The Aerococcus viridans L-lactate oxidase (avLOX) is a biotechnologically important member of this flavoenzyme family and it catalyzes oxidation of L-lactate and O2 into pyruvate and H2O2. Common characteristics of their structure are the (β/α)8 barrel fold and arrangement of protein subunits into a functional homotetramer2. The FMN is bound at the C-terminal end of the internal β barrel. A special and interesting feature of the catalytic center of avLOX is that it contains a third tyrosine (Tyr215), which forms a weak hydrogen bond with the pyruvate O2 in the wild-type structure.

Crystals of the Y215F mutant grew in the P21 spacegroup and had two tetramers within the asymmetric unit. Also present in each subunit is the FMN cofactor and a pyruvate which both bind in a similar manner to the wild-type enzyme. Residues 200–215 in subunit D and 200–216 in subunit H, which reside in loop 4 had no corresponding interpretable density. These residues form a short helical structure, which could function as an active-site lid, and residues near this range have been observed to be disordered in other structures suggesting an inherent mobility. In the six subunits with observable loop residues, the pyruvate is bound in a manner very similar to the wild-type enzyme except for a difference in the interaction with the amino acid at position 215. The interaction in the enzyme variant positions the nearest Phe215 ring atom within ~3.5 Å of the pyruvate methyl group to replace the hydrogen bond with a hydrophobic interaction. The hydrogen bond with Arg181 is also lost. In the two subunits without observable density for the loop, the pyruvate maintains some of the interactions between its carboxylate and Arg268 and Arg181 but shifts in the pyruvate and both of these side chains result in weaker interactions. The k5 of Y215F (20.3 s−1) at pH 6.5 was lowered 7-fold compared to the corresponding k5 of the wild-type enzyme (141 s−1). Evidence that k5 was nevertheless slowed down in the Y215F variant compared to wild-type enzyme at pH 6.5 could be explained by the development of new interactions between Phe215 and the bound pyruvate.

>[8x]MNNNDIEYNAPSEIKYIDVVNTYDLEEEASKVVPHGGFNYIAGASGDEWTKRANDRAWKHKLLYPRLAQDVEAPDTSTEILGHKIKAPFIMAPIAAHGLAHATKEAGTARAVSEFGTIMSISAYSGATFEEISEGLNGGPRWFQIYMAKDDQQNRDILDEAKGDGATAIILTADSTVSGNRDRDVKNKFVYPFGMPIVQRYLRGTAEGMSLNNIFGASKQKISPRDIEEIAAHSGLPVFVKGIQHPEDADMAIKAGASGIWVSNHGARQLYEAPGSFDTLPAIAERVNKRVPIVFDSGVRRGEHVAKALASGADVVALGRPVLFGLALGGWQGAYSVLDYFQKDLTRVMQLTGSQNVEDLKGLDLFDNPYGYEY> GSHMDSYELSPQLEELITKVSKAHQETFPSLCQLGKYTTNSSADHRVQLDLGLWDKFSELATKCIIKIVEFAKRLPGFTGLSIADQITLLKAACLDILMLRICTRYTPEQDTMTFSDGLTLNRTQMHNAGFGPLTDLVFAFAGQLLPLEMDDTETGLLSAICLICGDRMDLEEPEKVDKLQEPLLEALRLYARRRRPEQPYMFPRMLMKITDLRGISTKGAERAITLKMEIPGPMPPLIREMLENPEMFE

Retinoic Acid Receptors (RARs) belong to the large family of nuclear receptor proteins (NRs). RARs are ligand-dependent transcription factors involved in a plethora of cellular phenomena from embryonic development and organogenesis to homeostasis of most adult tissues. Forming heterodimers with Retinoid X Receptors (RXRs), RARs regulate the expression of several target genes via binding specific retinoic acid response elements (RARE). RARs display a common NR modular organization with mainly two structured domains, a central DNA binding domain (DBD), a C-terminal ligand binding domain (LBD), and an unstructured N-terminal domain (NTD).

To investigate the consequences of S371 phosphorylation, we crystallized a hRARγ LBD mutant bound to 9cis RA and C12m in which Ser371 is substituted by a Glu residue, which mimics a phosphorylated residue (hRARγS371E LBD). The complex crystallized into the P41212 with one monomer per asymmetric unit. The complex structure was solved by molecular replacement and refined to 1.7Å. The electron density map showed the presence of the ligand buried into the ligand-binding pocket and an extra electron density around position 371 confirmed the mutation of the serine residue into a glutamic acid. The detergent mediates a crystal contact in the region of the receptor involved in coactivator binding as described for the RARγ wild-type. The hRARγS371E and hRARγWT LBD structures are isomorphous and very similar with a Cα-RMSD of 0.47Å. The only notable difference between the two structures is the orientation of Arg387 in H10. Indeed, in RARγ wild-type R387 points towards the solvent, while in RARγS371E it forms a salt bridge with Asp340. Next, we investigated the effects of the S to E substitution on the region previously identified as the cyclin H binding site in RARα. This region is located over 40 Å from residue 371, and also shows a strong network of electrostatic interactions involving two salt bridges: one between R387 and D340 and another one between R341 and D269.>[6x]VGNKNNDKLTLWTTPDPSPNCKVSEEKDSKLTLVLTKCGSQILASVSLLVVKGKFANINNETNPGEDYKKFSVKLL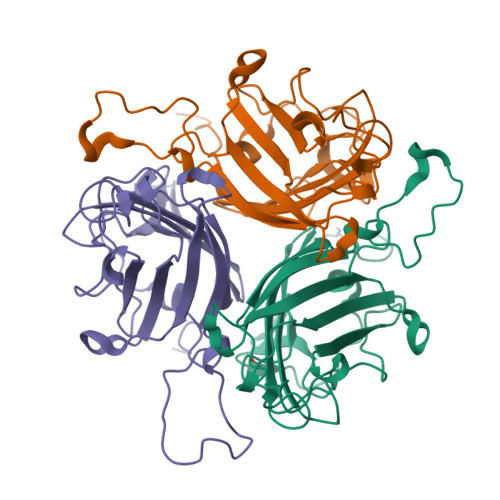FDANGKLLTGSSLDGNYWNYKNKDSVIGSPYENAVPFMPNSTAYPKIINNGTANPEDKKSAAKKTIVTNVYLGGDAGQPVATTVSFNKETESNCVYSITFDFAWNKTYKNVPFDSSSLTFSYIAQDAEDKNE> MITVDITVNDEGKVTDVIMDGHADHGEY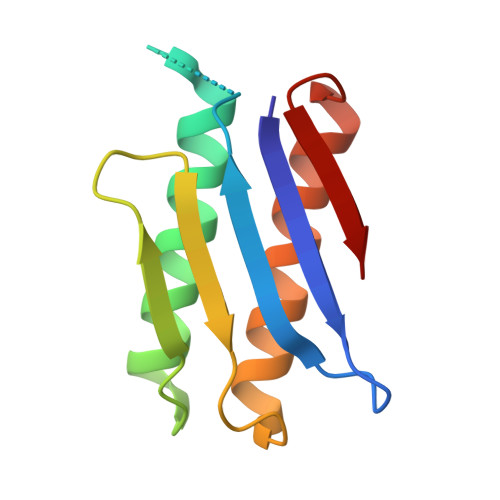GHDIVCAGASAVLFGSVNAIIGLTSERPDINYDDNGGHFHIRSVDTNNDEAQLILQTMLVSLQTIEEEYNENIRLNYK>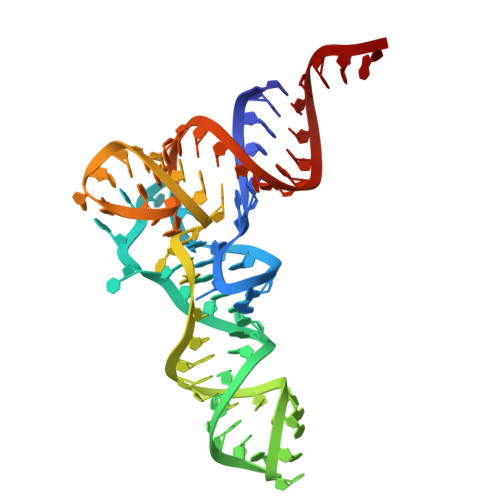 GGGCCCGUAGCUCAGUCUGGCAGAGCGCCUGGCUUUUAACCAGGUGGUCGAGGGUUCAAAUCCCUUCGGGCCCGCCA Bacterial microcompartments (BMC) are protein-based organelles that encapsulate enzymes participating in a given metabolic route. Thus, high resolution structures for several dozen shell subunits from different BMC types are now available. These data, combined with sequence information, confirmed that whilst differing in enzymatic contents, all BMC shells are built from homologous proteins adopting two structural folds. The first one (Pfam00936) is present in proteins that are organized as hexamers (BMC-H), and as tandem domains in subunits that form trimers (BMC-T). Here, we investigated this possibility by selecting the four CcmK paralogs that compose the shells of carboxysomes from the Synechocystis sp. PCC 6803 cyanobacteria (Syn6803).

The crystallization of K3/K4 hetero-hexamers was next attempted. We opted to increase K3/K4 abundance by means of pIsep-FPLC, a chromatofocusing-like purification approach. In that manner, the presumed His4-tagged K4 homo-hexamers could be removed, as indicated by the WB analysis of purified fractions that proved that most of FLAG signal was eluting with the second (most abundant) chromatographic peak. The pooled fractions collected for this peak were used for crystallographic assays. A condition resulted in a hexagonal crystal form diffracting X-rays to 1.80 Å resolution and displaying two molecules in the asymmetric unit. The only novel feature was the observation of a 2D arrangement with similarly-oriented K4 hexamers, which therefore differs from the stripped organization described before for the same protein, and provides an additional proof of the high structural plasticity of BMC-H proteins. CcmK3 absence in crystals prepared from samples of K4/K3 hetero-hexamers pointed to monomer rearrangements occurring during crystallization. The crystallization of CcmK4 from CcmK3/K4 samples might also point to a higher stability of homo-hexamers. Despite formation of 2D patches noticed in some experiments for K3/K4, the assemblies were smaller and less regular than those obtained with His4-tagged K4 homo-hexamers (right), which basically reproduced previous published results. In comparison, Tm of 89.2 and 62.3 °C were measured for K4 and K2, respectively, whereas fluorescence readings with the K1 homo-hexamer changed slowly and weakly with temperature, which prevented the determination of a Tm value.

>MAHHHHASGENLYFQGAMAAQSAVGSIETIGFPGILAAADAMVKAGRITIVGYIRAGSARFTLNIRGDVQEVKTAMAAGIDAINRTEGADVKTWVIIPRPHENVVAVLPIDFSPEVEPFREAAEGLNRRA[2x]>[2x]MSHQTGIQASEDVKEIFARARNGKYRLLKISIENEQLVVGSCSPPSDSWEQDYDSFVLPLLEDKQPCYVLFRLDSQNAQGYEWIFIAWSPDHSHVRQKMLYA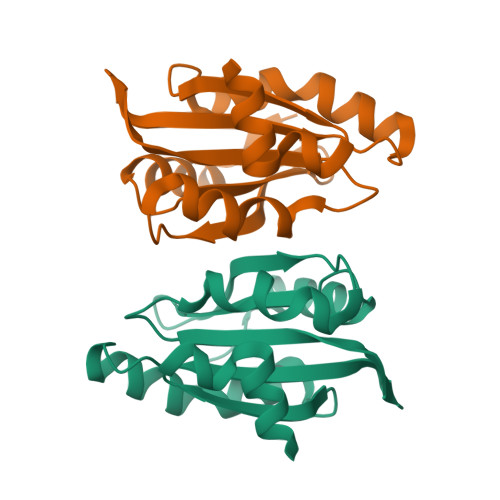ATRATLKKEFGGGHIKDEVFGTVKEDVSLHGYKKYLLSQS>GUAUAXAC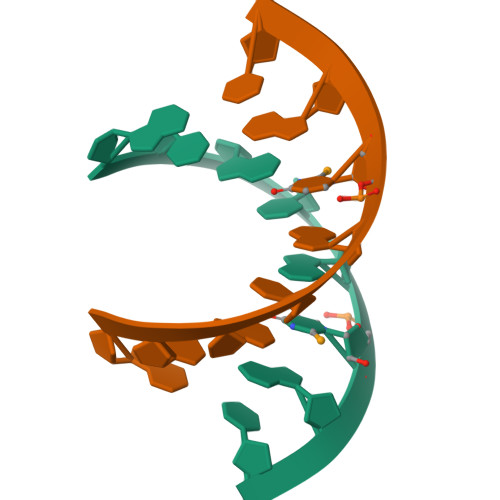[7x]2,2'-oxydiacetic acid 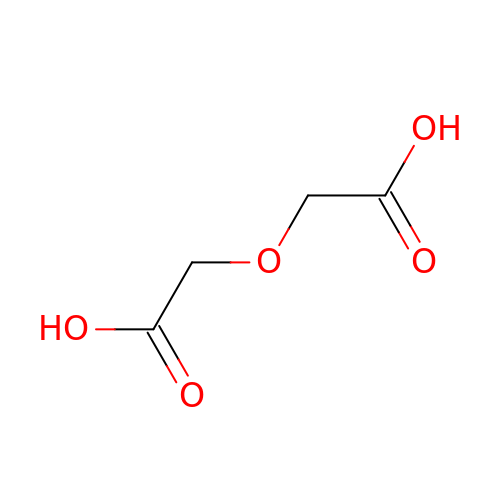| C4 H6 O5 | QEVGZEDELICMKH-UHFFFAOYSA-N> LVENVKQALFIPGQSCNKNLHDIMVDLSALKKPDMKRFNRKNDIHPFEDMSPLEFFSEKNDCSLMVLMTSSKKRKNNMTFIRTFGYKIYDMIELMVADNFKLLSDFKKLTFTVGLKPMFTFQGAAFDTHPVYKQIKSLFLDFFRGESTDLQDV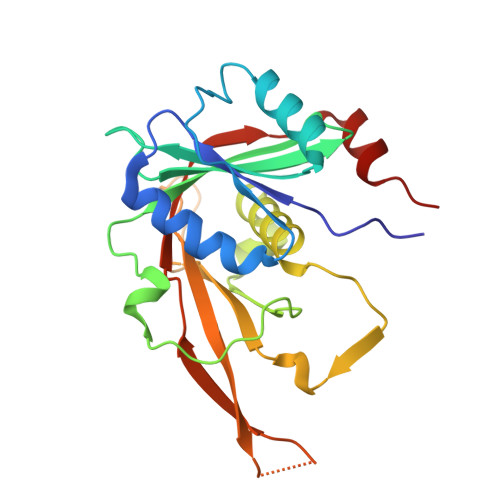AGLQHVISMTIQGDFQDGEPLPNVLFRVYKLKSYKSDQGGKRLPRIELVEIGPRLDFKIGRIHTPSPDMVTEAHKKP> MEIREGHNKFYINDKQGKQIAEIVFVPTGENLAIIEHTDVDESLKGQGIGKQLVAKVVEKMRREKRKIIPLCPFAKHEFDKTREYDD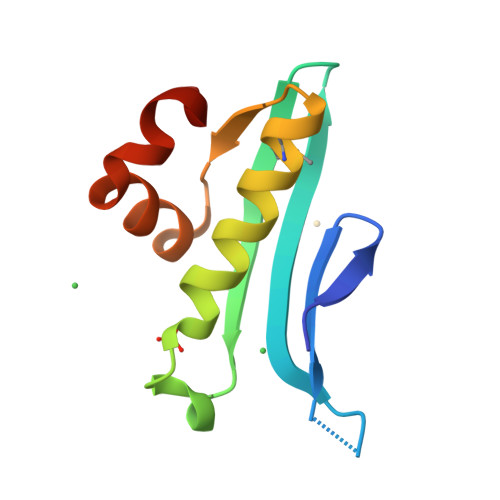IRSASN>[2x]MEFGFFDDANKEYVITVPRTPYPWINYLGTENFFSLISNTAGGYCFYRDARLRRITRYRYNNVPIDMGGRYFYIYDNGDFWSPGWSPVKRELESYECRHGLGYTKIAGKRNGIKAEVTFFVPLNYNGEVQKLILKNEGQDKKKITLFSFIEFCLWNAYDDMTNFQRNFSTGEVEIEGSVIYHKTEYRERRNHYAFYSVNAKISGFDSDRDSFIGLYNGFDAPQAVVNGKSNNSVADGWAPIASHSIEIELNPGEQKEYVFIIGYVENKDEEKWESKGVINKK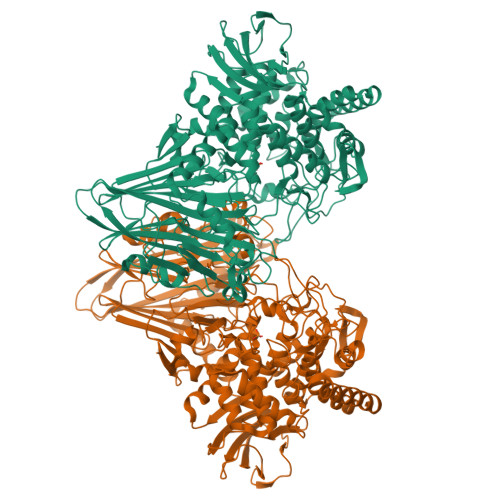KAYEMIEQFNTVEKVDKAFEELKSYWNALLSKYFLESHDEKLNRMVNIWNQYQCMVTFNMSRSASYFESGIGRGMGFRDSNQDLLGFVHQIPERARERLLDLAATQLEDGSAYHQYQPLTKKGNNEIGSNFNDDPLWLILATAAYIKETGDYSILKEQVPFNNDPSKADTMFEHLTRSFYHVVNNLGPHGLPLIGRADWNDCLNLNCFSTVPDESFQTTTSKDGKVAESVMIAGMFVFIGKDYVKLCEYMGLEEEARKAQQHIDAMKEAILKYGYDGEWFLRAYDDFGRKVGSKENEEGKIFIESQGFCVMAEIGLEDGKALKALDSVKKYLDTPYGLVLQNPAFTRYYIEYGEISTYPPGYKENAGIFCHNNAWIICAETVVGRGDMAFDYYRKIAPAYIEDVSDIHKLEPYVYAQMVAGKDAKRHGEAKNSWLTGTAAWNFVAISQWILGVKPDYDGLKIDPCIPKAWDGYKVTRYFRGSTYEITVKNPNHVSKGVAKITVDGNEISGNILPVFNDGKTHKVEVILEHHHHHH> GSEFSAKDERAREILRGFKLNWMNLRDAETGKILWQGTEDLSVPGVEHEARVPKKILKCKAVSRELNFSSTEQMEKFRLEQKVYFKGQCLEEWFFEFGFVIPNSTNTWQSLIEAAPESQMMPASVLTGNVIIETKFFDDDLLVSTSRVRLFYV

RAS is a major anticancer drug target which requires membrane localization to activate downstream signal transduction. Phosphodiesterase 6δ (PDE6D) has a beta-sandwich immunoglobulin fold which contains a hydrophobic pocket capable of binding to the farnesyl group. PDE6D binds to and sequesters the lipid of cytoplasmic RAS and has been proposed to deliver GTPase to recycling endosomes, which is followed by release mediated by the small G-protein Arf-like 2 (ARL2), allowing RAS to be trafficked back to the plasma membrane. The resultant lipid modification increases the affinity of RAS proteins toward membranes, where it is required for signal transduction. Here, we present a novel strategy for targeting RAS by stabilizing its interaction with the prenyl-binding protein PDE6D and disrupting its localization.

The only conserved feature is the modified C-terminal cysteine residue. Indeed, the affinities of 13-residue C-terminal peptides of WT KRAS and HRAS for PDE6D (1.3 and 2.7 μM, respectively) are comparable to those reported for full-length KRAS (1–2 μM)29 and RheB (∼0.5 μM). These affinities are also similar to those of a carboxymethylated geranylgeranylated cysteine residue (2.7 μM) and a carboxymethylated farnesylated cysteine residue (0.9 μM), suggesting that most residues preceding the lipidated cysteine do not affect binding to PDE6D. Interestingly, in addition to N/H/KRAS, more 4 farnesylated proteins, 10 geranylgeranylated, and 6-double geranylgeranylated binding partners were identified.>[2x]GSPGQDIQLIPPLINLLMSIEPDVIYAGHDNTKPDTSSSLLTSLNQLGERQLLSVVKWSKSLPGFRNLHIDDQITLIQYSWMSLMVFGLGWRSYKHVSGQMLYFAPDLILNEQRMKESSFYSLCLTMWQIPQEFVKLQVSQEEFLCMKVLLLLNTIPLEGLRSQTQFEEMRSSYIRELIKAIGLRQKGVVSSSQRFYQLTKLLDNLHDLV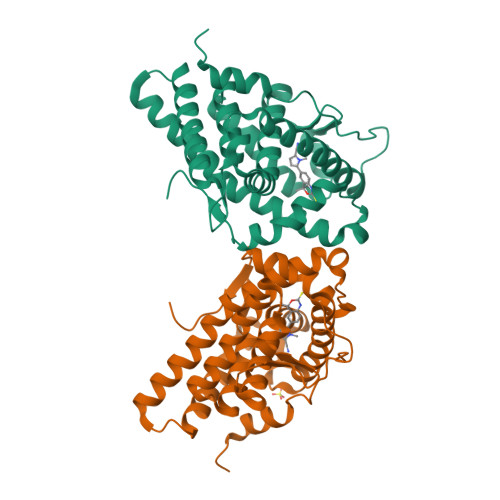KQLHLYCLNTFIQSRALSVEFPEMMSEVIAAQLPKILAGMVKPLLFHKK1,2,4-trimethylbenzene | C9 H12 | 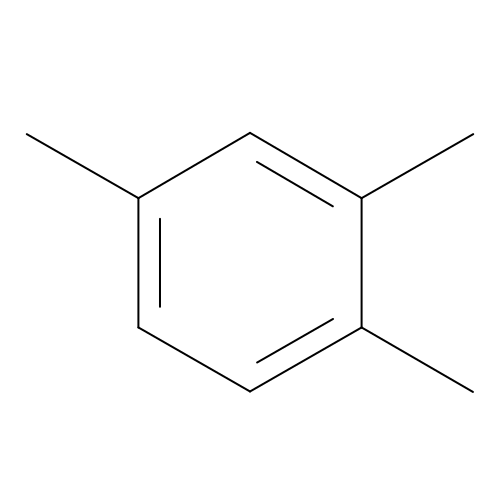GWHJZXXIDMPWGX-UHFFFAOYSA-N> MQRSPVEDANCLSRYFFWWTNPIMRKGFKEKLRPSDVYQAPSQDAADILAERLEKEWDREVASGKKKPSLLRAMARCYIKPFLLFGFLLYIGEATKTVQPQLLGRIIASFDPAHEPERANGYFLAFGLGLLFTARFLLLQPAMFGLHHLGMQIRIALFSIIYKKTLKLSSRVLDKISTGQLVSLMSANLGKFDQSLGMAHFIWISPLQCILCTGLIWELIDVNSFCALAAISLLGVLQAFLSHKMGPYKAQKVLLTNKRLALTSEIMENLHSVKAYGWEEIMETLIKNIRQDEVKLTRKIGSLRYFYSSAYFFSAIFVIVAAVVPHALSRGINLRRIFTTLSYCMVLRMTVTRQLPGSIQMWYDTMRLIWKIEEFLSKEEYKLMEYDLSITELELQDVTASWDEGPGELLERIKQENKANGHHNGDAGLFFTNLYVAPVLKDISLKLKKGEMLAVTGSMGSGKSSLLMTILGELVPSSGKIRHSGRISYSSQTAWIMPGTIRDNILFGLTYDEYRYKSVVKACQLEEDLAALPEKDKTPMAEGGLNLSGGQKARVALARAVYRDADLYLLDAPFTHLDIATEKEIFDKCLCKLMASKTRILVTNKIEHLKRADKILLLHNGESFFYGTFPELQSERPDFSSLLLGLEAYDNISAERRCSILTETLHRVSVDESAGMQPERSAFRQVPPTKPMYIDERKASVIVNPLGVARKASFIQVPEEEVRRTLPDRKFSLVPENELVDESFMGSDVYHNHGVHMAGQRRQSVLAFMTNAQGQGRREHLQSSFRRRLSVVPQSELASELDIYTRRLSDSTYDMTGILEEENIEACLTDEIDEIEETFETTKWNTYVRYVSNNKSLLYVLIFILFIAAIEIAGSVAGIFLITDELWREEHQRSEPNMTKHSNASSSGQTYAITVTPTSSYYILYIYVATSESLLAMGFFRGLPFVHTTITISKKLHQKMLHAVLSAPMSVLNTMKTGRIMNRFTKDMATIDDMLPLLMFDFVQLTVVVVGCILVVSIVRPYIFLAATPLAIIFIVMRKYFLRTGQQLKQLETEARSPIFSHLIMSLKGLWTIRAFERQAYFEALFHKTLNTHTATWFLYLSTLRWFLFRADILFVFFFTLAAWIAVGTNQDKPGEIGIIICLAMLILGTFQWCVATSIAVDGMMRSVDRVFKFIDLPSETPKPDKGKDSDLIIENVDAQADSSWPHRGQIEVRNLTVKYTEAGHAVLKNLSFSAEGRQRVGILGRTGSGKSSLFNALLKLVYTDGEISIDGVNWNKMPLQKWRKAFGVVPQKVFIFTGPLRMNLDPYGCHSDEELWRVAEEVGLKTVIEQFPDKLDFQLEYGGYVLSNGHKQLICLARSILSGARILLLDEPSAHLDPVTIKVLKKTLRQSFSTCT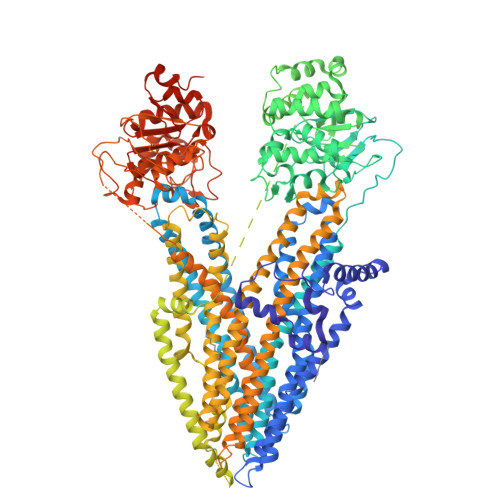ILLSEHKVEPLLECQSFLMMDKGQVKTYDSIQKLLNETSHLKQAISPAERLKLFPRRNSSMRTPQSKLSSVTQTLQEEAEDNIQDTRLSNSLEVLFQ[(4R,5R)-5-(hydroxycarbamoyl)-2,2-dimethyl-1,3-dioxolan-4-yl]methyl 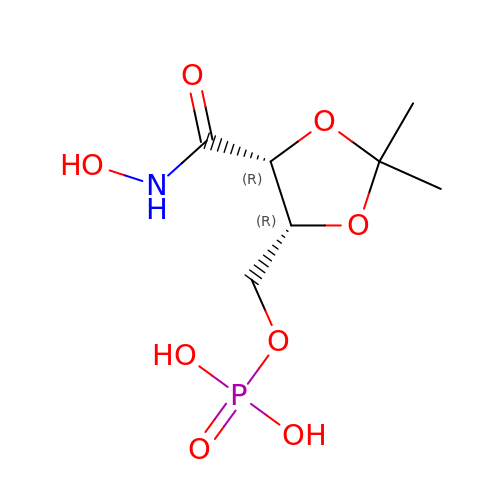dihydrogen phosphate | C7 H14 N O8 P | DVFAQEVWJBLFDS-RFZPGFLSSA-N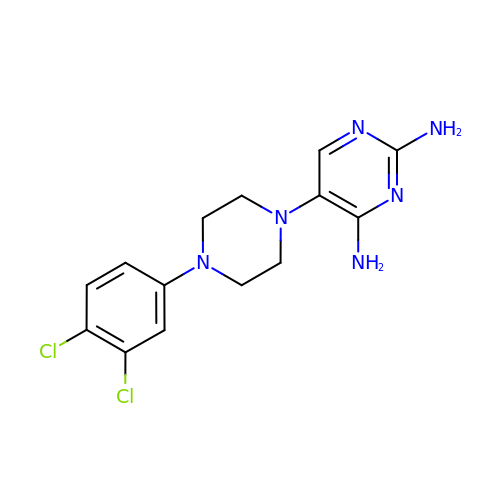5-[4-(3,4-dichlorophenyl)piperazin-1-yl]pyrimidine-2,4-diamine | C14 H16 Cl2 N6 | YYBKNWXCJMWHIP-UHFFFAOYSA-N> GAEFDLDQGGEALAPRQVLDLEDLVFTQGSHFMANKRCQLPDGSFRRQRKGYEEVHVPALKPKPFGSEEQLLPVEKLPKYAQAGFEGFKTLNRIQSKLYRAALETDENLLLCAPTGAGKTNVALMCMLREIGKHINMDGTINVDDFKIIYIAPMRSLVQEMVGSFGKRLATYGITVAELTGDHQLCKEEISATQIIVCTPEKWDIITRKGGERTYTQLVRLIILDEIHLLHDDRGPVLEALVARAIRNIEMTQEDVRLIGLSATLPNYEDVATFLRVDPAKGLFYFDNSFRPVPLEQTYVGITEKKAIKRFQIMNEIVYEKIMEHAGKNQVLVFVHSRKETGKTARAIRDMCLEKDTLGLFLREGSASTEVLRTEAEQCKNLELKDLLPYGFAIHHAGMTRVDRTLVEDLFADKHIQVLVSTATLAWGVNLPAHTVIIKGTQVYSPEKGRWTELGALDILQMLGRAGRPQYDTKGEGILITSHGELQYYLSLLNQQLPIESQMVSKLPDMLNAEIVLGNVQNAKDAVNWLGYAYLYIRMLRSPTLYGISHDDLKGDPLLDQRRLDLVHTAALMLDKNNLVKYDKKTGNFQVTELGRIASHYYITNDTVQTYNQLLKPTLSEIELFRVFSLSSEFKNITVREEEKLELQKLLERVPIPVKESIEEPSAKINVLLQAFISQLKLEGFALMADMVYVTQSAGRLMRAIFEIVLNRGWAQLTDKTLNLCKMIDKRMWQSMCPLRQFRKLPEEVVKKIEKKNFPFERLYDLNHNEIGELIRMPKMGKTIHKYVHLFPKLELSVHLQPITRSTLKVELTITPDFQWDEKVHGSSEAFWILVEDVDSEVILHHEYFLLKAKYAQDEHLITFFVPVFEPLPPQYFIRVVSDRWLSCETQLPVSFRHLILPEKYPPPTELLDLQPLPVSALRNSAFESLYQDKFPFFNPIQTQVFNTVYNSDDNVFVGAPTGSGKTICAEFAILRMLLQSSEGRCVYITPMEALAEQVYMDWYEKFQDRLNKKVVLLTGETSTDLKLLGKGNIIISTPEKWDILSRRWKQRKNVQNINLFVVDEVHLIGGENGPVLEVICSRMRYISSQIERPIRIVALSSSLSNAKDVAHWLGCSATSTFNFHPNVRPVPLELHIQGFNISHTQTRLLSMAKPVYHAITKHSPKKPVIVFVPSRKQTRLTAIDILTTCAADIQRQRFLHCTEKDLIPYLEKLSDSTLKETLLNGVGYLHEGLSPMERRLVEQLFSSGAIQVVVASRSLCWGMNVAAHLVIIMDTQYYNGKIHAYVDYPIYDVLQMVGHANRPLQDDEGRCVIMCQGSKKDFFKKFLYE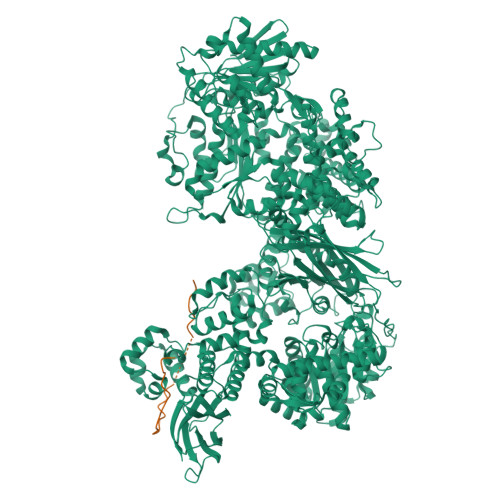PLPVESHLDHCMHDHFNAEIVTKTIENKQDAVDYLTWTFLYRRMTQNPNYYNLQGISHRHLSDHLSELVEQTLSDLEQSKCISIEDEMDVAPLNLGMIAAYYYINYTTIELFSMSLNAKTKVRGLIEIISNAAEYENIPIRHHEDNLLRQLAQKVPHKLNNPKFNDPHVKTNLLLQAHLSRMQLSAELQSDTEEILSKAIRLIQACVDVLSSNGWLSPALAAMELAQMVTQAMWSKDSYLKQLPHFTSEHIKRCTDKGVESVFDIMEMEDEERNALLQLTDSQIADVARFCNRYPNIELSYEVVDKDSIRSGGPVVVLVQLEREEEVTGPVIAPLFPQKREEGWWVVIGDAKSNSLISIKRLTLQQKAKVKLDFVAPATGAHNYTLYFMSDAYMGCDQEYKFSVDVKEA;> GAMAFNPHTSDLPSSKVNENSLGTLDESKSSDSHSDSDGEQEAEEGGVSTETEKPKIKFKEKNKNSDGGSDPETQKEKSIQKQNSLGSNEEKSKTLKKSNPYGEWQEIKQEVESHEEVDLELPSTENEYVSTSEADGGGEPKVVFKEKTVTSLGVMADGVAPVFKKRRTENGKSRNLRQRGDDQ(1S,2S)-N'-(chloroacetyl)-2-phenylcyclopropane-1-carbohydrazide | C12 H13 Cl N2 O2 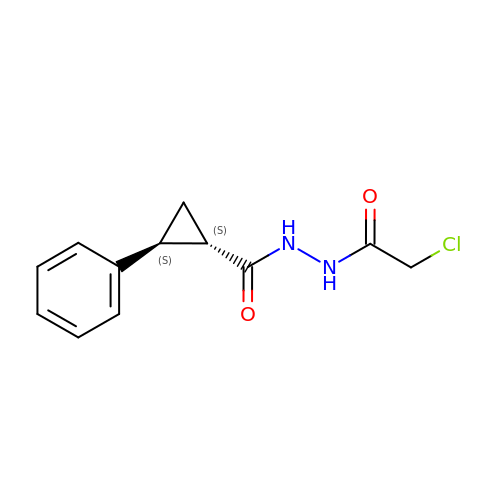| MDZKSIJGAAFPGQ-ZJUUUORDSA-N> AYSNTYQEFTNIDQAKAWGNAQYKKYGLSKSEKEAIVSYTKSASEINGKLRQNKGVINGFPSNLIKQVELLDKSFNKMKTPENIM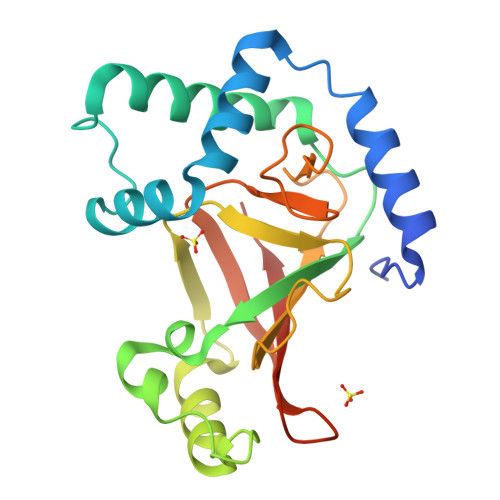LFRGDDPAYLGTEFQNTLLNSNGTINKTAFEKAKAKFLNKDRLEYGYISTSLMNVSQFAGRPIITKFKVAKGSKAGYIDPISAFAGALEMLLPRHSTYHIDDMRLSSDGKQIIITATMMGTAINPK>MEAIVGKVTEVNKDTFWPIVKAAGDKPVVLDMFTQWCGPCKAMAPKYEKLAEEYLDVIFLKLDCNQENKTLAKELGIRVVPTFKILKENSVVGEVTGAKYDKLLEAIQAARS[2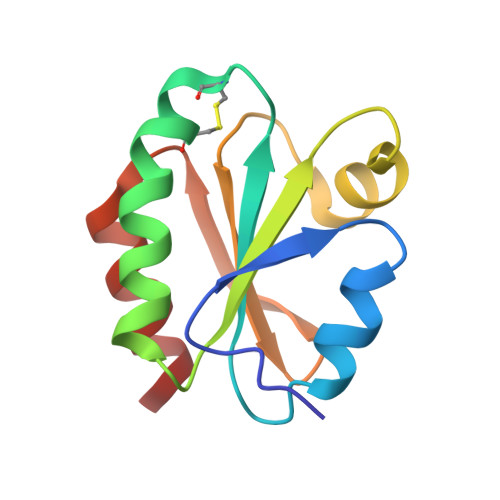x]>KYLLSPETIEALRKPTFDVWLWEPNEMLSCLEHMYHDLGLVRDFSINPVTLRRWLFCVHDNYRNNPFHNFRHCFCVAQMMYSMVWLCSLQEKFSQTDILILMTAAICHDLDHPGYNNTYQINARTELAVRYNDISPLENHHCAVAFQILAEPECNIFSNIPPDGFKQIRQGMITLILATDMARHAEIMDSFKEKMENFDYSNEEHMTLLKMILIKCCDISNEVRPMEVAEPWVDCLLEEYFMQSDREKSEGLPVAPFMDRDKVTKATAQIGFIKFV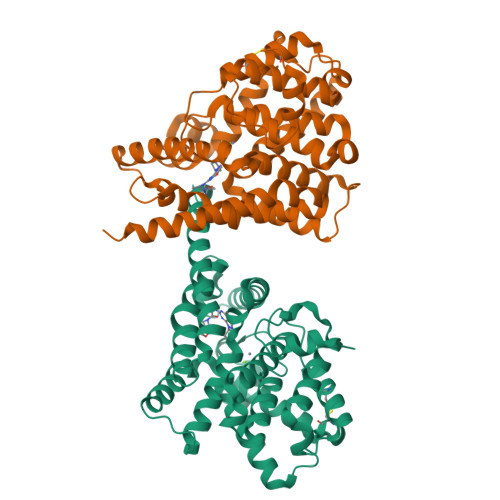LIPMFETVTKLFPMVEEIMLQPLWESRDRYEELKRIDDAMKELQKK[2x]> GNMEAS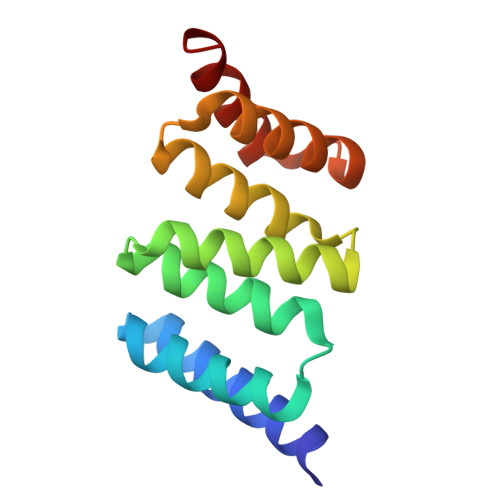EVMKEKGNAAYKGKQWNKAVNFYTEAIKLNGANATYYCNRAAAFLELCCFQQAEQDCTKAMLIDKKNVKAYLRRGTARESLVRYKEAAADFRHALVLEPQNKTAKVAEKRLRKHI>KDWTQYVNPLMGSQSTFELSTGNTYPAIARPWGMNFWTPQTGKMGDGWQYTYTANKIRGFKQTHQPSPWINDYGQFSIMPIVGQPVFDEEKRASWFAHKGEVATPYYYKVYLAEHDIVTEMTPTERAVLFRFTFPENDHSYVVVDAFDKGSYIKIIPEENKIIGYTTRNSGGVPENFKNYFIIEFDKPFTYKATVENGNLQENVAEQTTDHAGAIIGFKTRKGEQVNARIASSFISFEQAAANMNELGKDNIEQLAQKGKDAWNQVLGKIEVEGGNLDQYRTFYSCLYRSLLFPRKFYELDANGQPIHYSPYNGQVLPGYMFTDTGFWDTFRCLFPLLNLMYPSVNKEMQEGLINTYLESGFFPEWASPGHRGCMVGNNSASILVDAYMKGVKVDDIKTLYEGLIHGTENVHPEVSSTGRLGYEYYNKLGYVPYDVKINENAARTLEYAYDDWCIYRLAKELKRPKKEISLFAKRAMNYKNLFDKESKLMRGRNEDGTFQSPFSPLKWGDAFTEGNSWHYTWSVFHDPQGLIDLMGGKEMFVTMMDSVFAVPPIFDDSYYGQVIHEIREMTVMNMGNYAHGNQPIQHMIYLYDYAGQPWKAQYWLRQVMDRMYTPGPDGYCGDEDNGQTSAWYVFSALGFYPVCPGTDEYVMGTPLFKKATLHFENGNSLVIDAPNNSTENFYIDSMSFNGADHTKNYLRHEDLF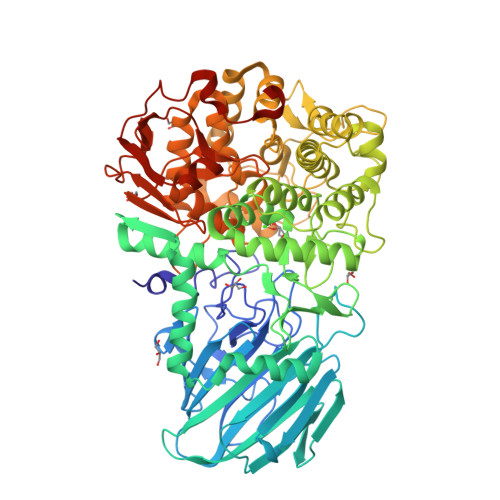KGGTIKVDMSNRPNLNRGTKEEDMPYSFSKELEHHHHHH[8x]> MRRFALTVALPKGRMFREAYEVLKRAGLDLPEVEGERTLLHGKEGGVALLELRNKDVPIYVDLGIAEIGVVGKDVLLDSGRDLFEPVDLGFGACRLSLIRRPGDTGPIRRVATKYPNFTARLLKERGWAAD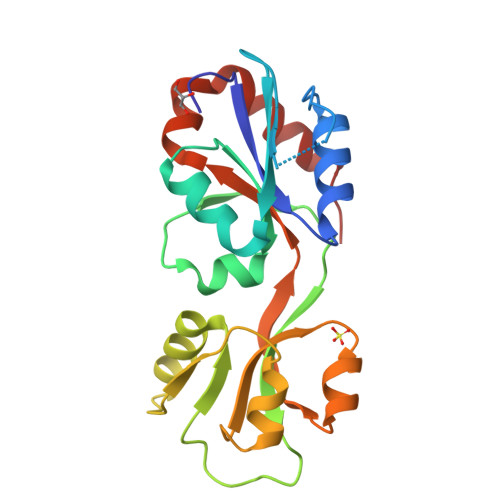VVELSGNIELAAVTGLADAVVDVVQTGATLRAAGLVEVEVLAHSTARLVVNRQALKLKRAVLKPLIQRLRELSGS>SNAMTLLDGKALSAKIKEELKEKNQFLKSKGIESCLAVILVGDNPASQTYVKSKAKACEECGIKSLVYHLNENITQNELLALINTLNHDDSVHGILVQLPLPDHICKDLILESIISSKDVDGFHPINVGYLNLGLESGFLPCTPLGVMKLLKAYEIDLEGKDAVIIGASNIVGRPMATMLLNAGATVSVCHIKTKDLSLYTRQADLIIVAAGCVNLLRSDMVKEGVIVVDVGINRLESGKIVG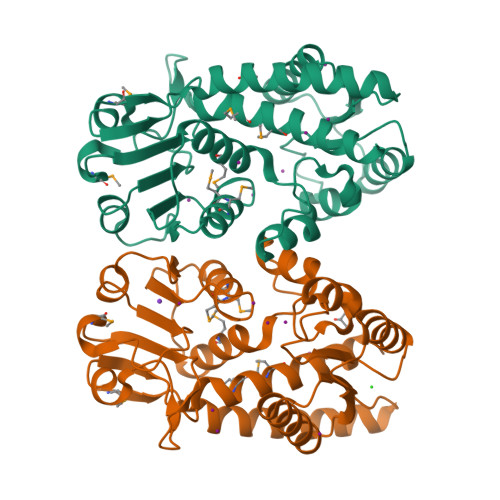DVDFEEVSKKSSYITPVPGGVGPMTIAMLLENTVKSAKNRLN[2x]The ABC transporter CydDC plays a central role in the biogenesis of membrane-integrated and soluble cytochromes. Here, we used cellular, biochemical, structural and computational methods to characterize the structure and function of the heterodimeric bacterial ABC transporter CydDC. We provide multi-level evidence that CydDC is a heme transporter required for functional maturation of cytochrome bd, a pharmaceutically relevant drug target. Each subunit is composed of a membrane domain formed by six transmembrane α-helices (TMH), an N-terminal cytoplasmic elbow helix oriented parallel to the membrane plane and a cytoplasmic NBD.

Based on the deduced sequence of binding events and the distinct interaction patterns between heme and CydDC, we reasoned that the interaction between H85C and the heme iron marks the most crucial step of substrate recognition. To test this hypothesis, we generated a CydDC H85AC mutant and performed growth-restoring complementation studies and oxygen consumption measurements. In addition, we investigated the effect of the histidine to alanine replacement on ATP hydrolysis activity. A lack of this highly conserved histidine residue abrogates the functionality of CydDC. Furthermore, CydDCH85A could not be copurified with bound heme and could not be loaded by the exogenous addition of heme. These observations were confirmed by cryo-EM structures of CydDCH85A, exclusively adopting the IFasisolatedapo conformation, irrespective of presence or absence of exogenously added heme to the samples.

> MRALLPYLALYKRHKWMLSLGIVLAIVTLLASIGLLTLSGWFLSASAVAGVAGLYSFNYMLPAAGVRGAAITRTAGRYFERLVSADATFRVLQHLRIYTFSKLLPLSPAGLARYRQGELLNRVVADVDTLDHLYLRVISPLVGAFVVIMVVTIGLSFLDFTLAFTLGGIMLLTLFLMPPLFYRAGKSTGQNLTHLRGQYRQQLTAWLQGQAELTIFGASDRYRTQLENTEIQWLEAQRRQSELTALSQAIMLLIGALAVILMLWMASGGVGGNAQPGALIALFVFCALAAFEALAPVTGAFQHLGQVIASAVRISDLTDQKPEVTFPDTQTRVADRVSLTLRDVQFTYPEQSQQALKGISLQVNAGEHIAILGRTGCGKSTLLQQLTRAWDPQQGEILLNDSPIASLNEAALRQTISVVPQRVHLFSATLRDNLLLASPGSSDEALSEILRRVGLEKLLEDAGLNSWLGEGGRQLSGGELRRLAIARALLHDAPLVLLDEPTEGLDATTESQILELLAEMMREKTVLMVTHRLRGLSRFQQIIVMDNGQIIEQGTHAELLARQGRYYQFKQGL;> MNKSRQKELTRWLKQQSVISQRWLNISRLLGFVSGILIIAQAWFMARILQHMIMENIPREALLLPFTLLVLTFVLRAWVVWLRERVGYHAGQHIRFAIRRQVLDRLQQAGPAWIQGKPAGSWATLVLEQIDDMHDYYARYLPQMALAVSVPLLIVVAIFPSNWAAALILLGTAPLIPLFMALVGMGAADANRRNFLALARLSGHFLDRLRGMETLRIFGRGEAEIESIRSASEDFRQRTMEVLRLAFLSSGILEFFTSLSIALVAVYFGFSYLGELDFGHYDTGVTLAAGFLALILAPEFFQPLRDLGTFYHAKAQAVGAADSLKTFMETPLAHPQRGEAELASTDPVTIEAEELFITSPEGKTLAGPLNFTLPAGQRAVLVGRSGSGKSSLLNALSGFLSYQGSLRINGIELRDLSPESWRKHLSWVGQNPQLPAATLRDNVLLARPDASEQELQAALDNAWVSEFLPLLPQGVDTPVGDQAARLSVGQAQRVAVARALLNPCSLLLLDEPAASLDAHSEQRVMEALNAASLRQTTLMVTHQLEDLADWDVIWVMQDGRIIEQGRYAELSVAGGPFATLLAHRQEEI> MKILVIGPSWVGDMMMS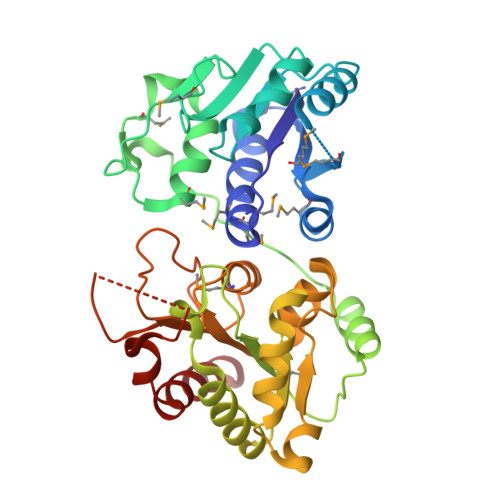QSLYRTLQARYPQAIIDVMAPAWCRPLLSRMPEVNEAIPMPLGHGALEIGERRKLGHSLREKRYDRAYVLPNSFKSALVPLFAGIPHRTGWRGEMRYGLLNDVRVLDKEAWPLMVERYIALAYDKGIMRTAQDLPQPLLWPQLQVSEGEKSYTCNQFSLSSERPMIGFCPGAEFGPAKRWPHYHYAELAKQLIDEGYQVVLFGSAKDHEAGNEILAALNTEQQAWCRNLAGETQLDQAVILIAACKAIVTNDSGLMHVAAALNRPLVALYGPSSPDFTPPLSHKARVIRLITGYHKVRKGDAAEGYHQSLIDITPQRVLEELNALLLQEEA PIEZO channels transmit mechanical force signals to cells, allowing them to make critical decisions during development and in pathophysiological conditions. Here, we report several near-atomic resolution cryo-EM structures of fast-inactivating wild-type human PIEZO1 (hPIEZO1) and its slow-inactivating channelopathy mutants with or without its auxiliary subunit MDFIC. Each hPIEZO1 subunit has a curved blade structure, and the three subunits form the trimeric PIEZO channel, exhibiting a bowl-like shape. MDFIC, a MyoD family inhibitor protein, has recently been identified as an auxiliary subunit of piezo channels capable of decelerating channel inactivation and attenuating channel mechanosensitivity.

We selected the mild GOF mutants hPIEZO1-A1988V and hPIEZO1-E756del, familiar in African populations with a slightly longer inactivation time, and the more severe R2456H mutant with a much longer inactivation time. The E756del mutation is located at the THU4 and THU5 linker, the A1988V mutation is located at the THU9 linker, and the R2456H mutation is located at the IH of the pore module. At the same time, the channelopathy mutants A1988V, E756del, and R2456H present a slow inactivation rate with half inactivation time of 13.4±3.8 ms, 18.5±4.1 ms, and 23.2±2.9 ms, respectively. We then tried and obtained almost twice as many hPIEZO1-A1988V images as the wild type but only achieved a 3.7 Å resolution cryo-EM density map. Yet, the resulting overall structure is similar to the wild type. Based on these results, these three hPIEZO1 channelopathy GOF mutants may be structurally less stable than wild type. However, in the mild GOF hPIEZO1-A1988V, which has a slower inactivation rate compared to wild-type hPIEZO1, the acyl chains of the pore lipid are retracted from the central hydrophobic pore to the side of the IH, although the hydrophilic phosphate group heads still interact with R2456. Consistently, the slower inactivating hPIEZO1-A1988V mutant has the same hydrophobic acyl chain tails retracted from the hydrophobic pore region, implying that the pore lipids are involved in the fast inactivation of hPIEZO1. Mild channelopathy mutants or mPIEZO1 show the pore lipids retracted from the pore and thus exhibit a slow inactivation pattern.

>[3x]ELVKGVYAKYWIYVCAGMFIVVSFAGRLVVYKIVYMFLFLLCLTLFQVYYSLWRKLLKAFWWLVVAYTMLVLIAVYTFQFQDFPAYWRNLTGFTDEQLGDLGLEQFSVSELFSSILVPGFFLLACILQLHYFHRPFMQLTDMEHVSLPGTRLPRWAHRQDAVSGTPLLREEQQEHQQQQQEEEEEEEDSRDEGLGVATPHQATQVPEGAAKWGLVAERLLELAAGFSDVLSRVQVFLRRLLELHVFKLVALYTVWVALKEVSVMNLLLVVLWAFALPYPRFRPMASCLSTVWTCVIIVCKMLYQLKVVNPQEYSSNCTEPFPNSTNLLPTEISQSLLYRGPVDPANWFGVRKGFPNLGYIQNHLQVLLLLVFEAIVYRRQEHYRRQHQLAPLPAQAVFASGTRQQLDQDLLGCLKYFINFFFYKFGLEICFLMAVNVIGQRMNFLVTLHGCWLVAILTRRHRQAIARLWPNYCLFLALFLLYQYLLCLGMPPALCIDYPWRWSRAVPMNSALIKWLYLPDFFRAPNSTNLISDFLLLLCASQQWQVFSAERTEEWQRMAGVNTDRLEPLRGEPNPVPNFIHCRSYLDMLKVAVFRYLFWLVLVVVFVTGATRISIFGLGYLLACFYLLLFGTALLQRDTRARLVLWDCLILYNVTVIISKNMLSLLACVFVEQMQTGFCWVIQLFSLVCTVKGYYDPKEMMDRDQDCLLPVEEAGIIWDSVCFFFLLLQRRVFLSHYYLHVRADLQATALLASRGFALYNAANLKSIDFHRRIEEKSLAQLKRQMERIRAKQEKHRQGRVDRSRPQDTLGPKDPGLEPGPDSPGGSSPPRRQWWRPWLDHATVIHSGDYFLFESDSEEEEEAVPEDPRPSAQSAFQLAYQAWVTNAQAVLRRRQQEQEQARQEQAGQLPTGGGPSQEVEPAEGPEEAAAGRSHVVQRVLSTAQFLWMLGQALVDELTRWLQEFTRHHGTMSDVLRAERYLLTQELLQGGEVHRGVLDQLYTSQAEATLPGPTEAPNAPSTVSSGLGAEEPLSSMTDDMGSPLSTGYHTRSGSEEAVTDPGEREAGASLYQGLMRTASELLLDRRLRIPELEEAELFAEGQGRALRLLRAVYQCVAAHSELLCYFIIILNHMVTASAGSLVLPVLVFLWAMLSIPRPSKRFWMTAIVFTEIAVVVKYLFQFGFFPWNSHVVLRRYENKPYFPPRILGLEKTDGYIKYDLVQLMALFFHRSQLLCYGLWDHEEDSPSKEHDKSGEEEQGAEEGPGVPAATTEDHIQVEARVGPTDGTPEPQVELRPRDTRRISLRFRRRKKEGPARKGAAAIEAEDREEEEGEEEKEAPTGREKRPSRSGGRVRAAGRRLQGFCLSLAQGTYRPLRRFFHDILHTKYRAATDVYALMFLADVVDFIIIIFGFWAFGKHSAVTDITSSLSDDQVPEAFLVMLLIQFSTMVVDRALYLRKTVLGKLAFQVALVLAIHLWMFFILPAVTERMFNQNVVAQLWYFVKCIYFALSAYQIRCGYPTRILGNFLTKKYNHLNLFLFQGFRLVPFLVELRAVMDWVWTDTTLSLSSWMCVEDIYANIFIIKCSRETEKKYPQPKGQKKKKIVKYGMGGLIILFLIAIIWFPLLFMSLVRSVVGVVNQPIDVTVTLKLGGYEPLFTMSAQQPSIIPFTAQAYEELSRQFDPQPLAMQFISQYSPEDIVTAQIEGSSGALWRISPPSRAQMKRELYNGTADITLRFTWNFQRDLAKGGTVEYANEKHMLALAPNSTARRQLASLLEGTSDQSVVIPNLFPKYIRAPNGPEANPVKQLQPNEEADYLGVRIQLRREQGAGATGFLEWWVIELQECRTDCNLLPMVIFSDKVSPPSLGFLAGYGIMGLYVSIVLVIGKFVRGFFSEISHSIMFEELPCVDRILKLCQDIFLVRETRELELEEELYAKLIFLYRSPETMIKWTREKE> GCG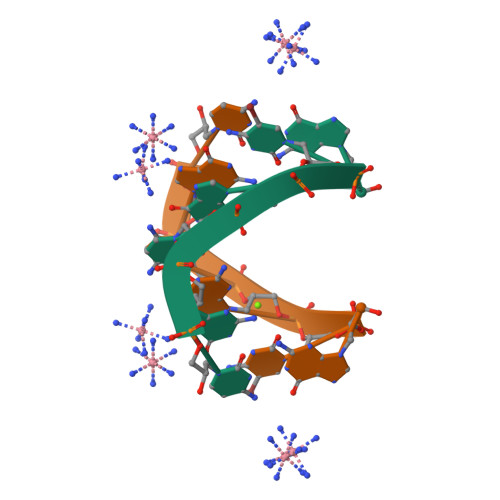CGC>[2x]MLELLPTAVEGVSQAQITGRPEWIWLALGTALMGLGTLYFLVKGMGVSDPDAKKFYAITTLVPAIAFTMYLSMLLGYGLTMVPFGGEQNPIYWARYADWLFTTPLLLLDLALLVDADQGTILALVGADGIMIGTGLVGALTKVYSYRFVWWAISTAAMLYILYVLFFGFTSKAESMRPEVASTFKVLRNVTVVLWSAYPVVWLIGSEGAGIVPLNIETLLFMVLDVSAKVGFGLILLR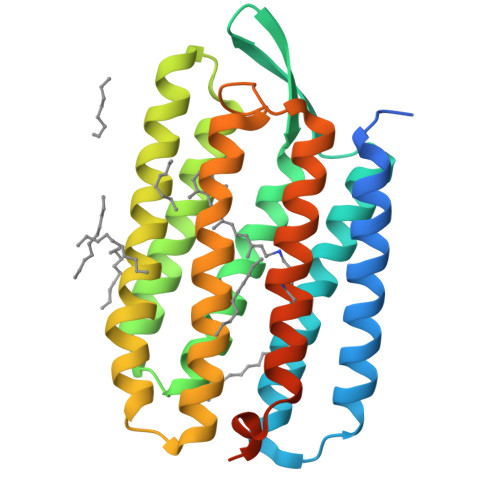SRAIFGEAEAPEPSAGDGAAATSD>SLELWLNKATDPSMSEQDWSAIQNFCEQVNTDPNGPTHAPWLLAHKIQSPQEKEALYALTVLEMCMNHCGEKFHSEVAKFRFLNELIKVLSPKY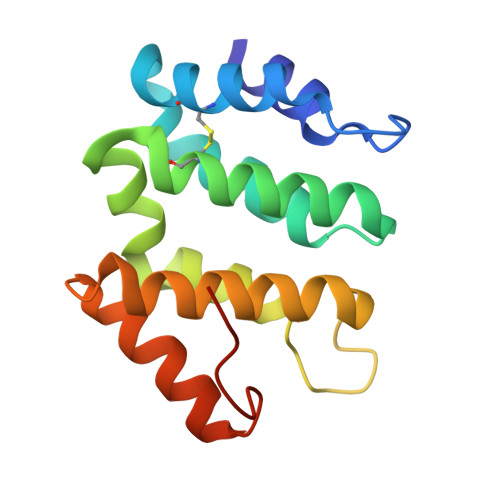LGSWATGKVKGRVIEILFSWTVWFPEDIKIRDAYQMLKKQGIIKQDPKLPVDKI[2x]>[2x]VINLDMIKASYITMGYDKNAAEVGEIIKATVKINKITNFSGYQVNIKYDPT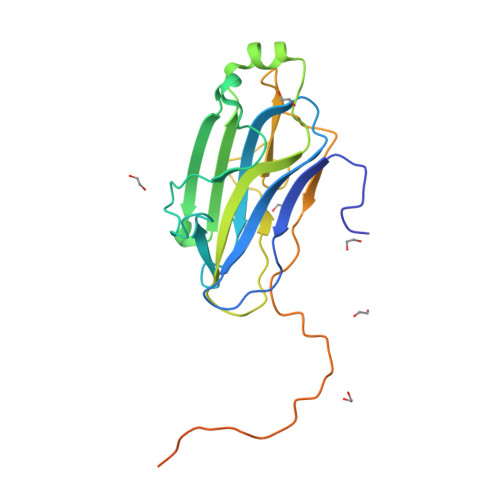VLQAVNPKTGVAYTNSSLPTSGELLVSEDYGPIVQGVHKISEGILNLSRSYTALEVYRASESPEETGTLAVVGFKVLQKKATTVVFEDSETMPNGITGTTLFNWYGNRIQSGYFVIQPGEINSAPIATATPTTKPTAFASTMPTVTLTPTPTATTTTTIPTAVPTTESLEHHHHHH>SMVLQPGDRVTHDKYGLGRVEEVAGTGESAMSLIDFGS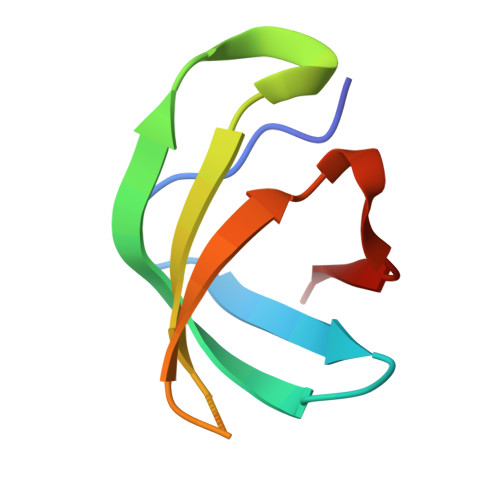AGRVKLMHNHAPLQKL[5x]> GPVAVTLHNEAITYTADITVGSDNQKLNVIVDTGSSDLWIPDSNVICIPKWRGDKGDFCKSAGSYSPASSRTSQNLNTRFDIKYGDGSYAKGKLYKDTVGIGGVSVRDQLFANVWSTSARKGILGIGFQSGEATEFDYDNLPISLRNQGIIGKAAYSLYLNSAEASTGQIIFGGIDKAKYSGSLVDLPITSEKKLTVGLRSVNVR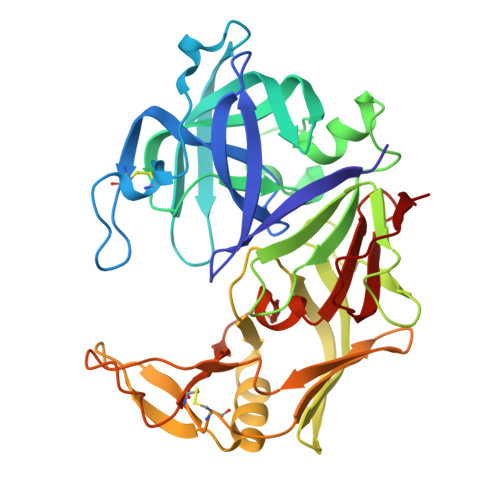GRNVDANTNVLLDSGTTISYFTRSIVRNILYAIGAQMKFDSAGNKVYVADCKTSGTIDFQFGNNLKISVPVSEFLFQTYYTSGKPFPKCEVRIRESEDNILGDNFLRSAYVVYNLDDKKISMAPVKYTSESDIVAIN1-[3-(2,3-dichlorophenoxy)propoxy]-6,6-dimethyl-1,6-dihydro-1,3,5-triazine-2,4-diamine 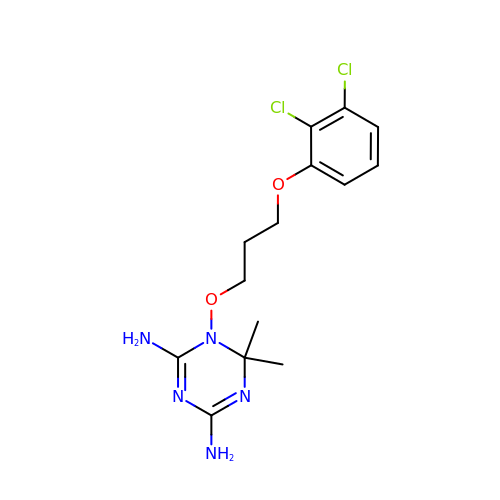| C14 H19 Cl2 N5 O2 | ZEXYNHJGHHPEOL-UHFFFAOYSA-N> MSRQASRLDAKKVNSEFLTLTYGALVTQMLRDFENAEDVNKQLERIGYNMGMRLIEDFLARTSAPRCLEMRETADRIQQAF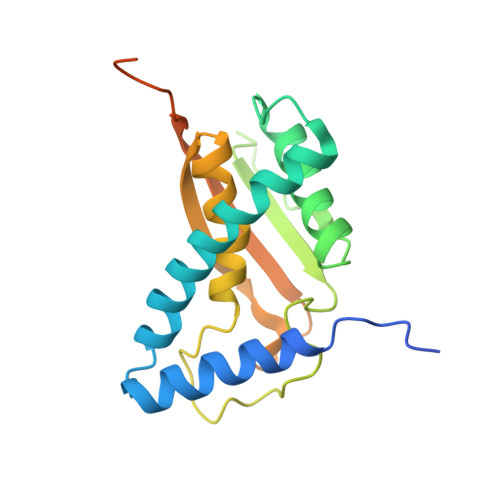RIYLNIQPTISNWSPASDEFSLVFDSNPLTEFVELPPDLTNLRYSAILSGCIRGALEMVQLEVQCWFVQDQLKGDNVTELRVKFVRRLEEVIPAGEDLEVLFQGPVASWSHPQFEKGAV1-benzyl-4-methoxybenzene | C14 H14 O | 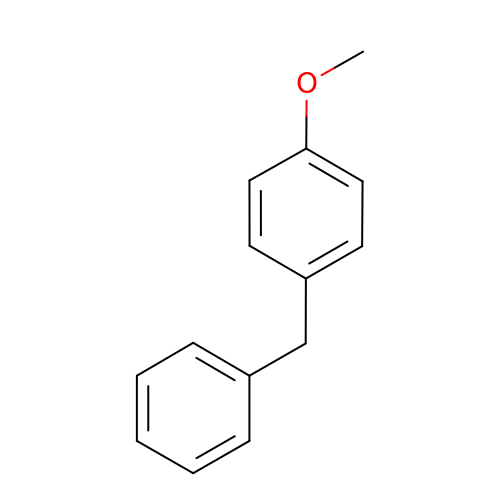GQLYCRTUQGSDSM-UHFFFAOYSA-N>GSHMSTGEAIPRVAVVVFILNG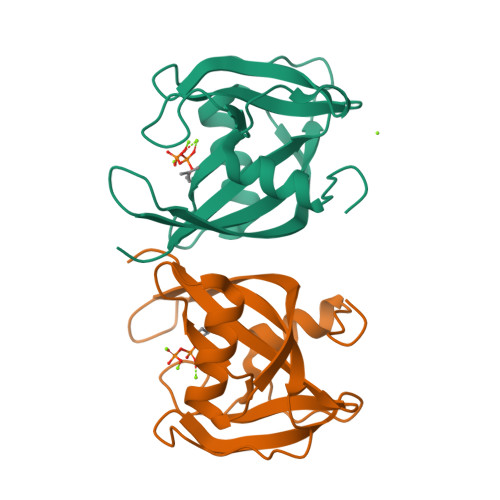NSILLGRRRSSIGNSTFALPGGHLEFGESFEECAAREVMEETGLKIEKMKLLTVTNNVFKEAPTPSHYVSVSIRAVLVDPSQEPKNMEPEKCEGWDWYDWENLPKPLFWPLEKLFGSGFNPFTHGGGD[2x]> SMGKKSRVKTQKSGTGATATVSPKEILNLTSELLQKCSSPAPGPGKEWEEYVQIRTLVEKIRKKQKGLSVTFDGKREDYFPDLMKWASENGASVEGFEMVNFKEEGFGLRATRDIKAEELFLWVPRKLLMTVESAKNSVLGPLYSQDRILQAMGNIALAFHLLCERASPNSFWQPYIQTLPSEYDTPLYFEEDEVRYLQSTQAIHDVFSQYKNTARQYAYFYKVIQTHPHANKLPLKDSFTYEDYRWAVSSVMTRQNQIPTEDGSRVTLALIPLWDMCNHTNGLITTGYNLEDDRCECVALQDFRAGEQIYIFYGTRSNAE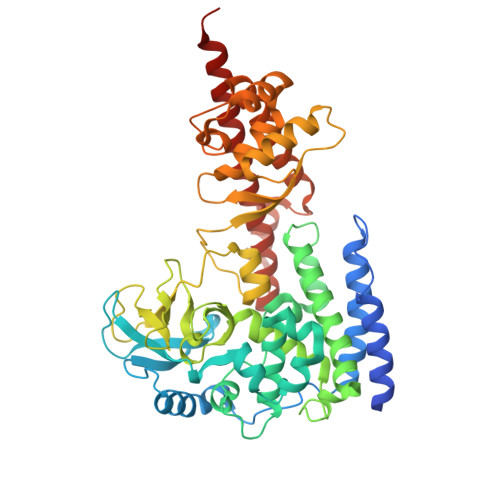FVIHSGFFFDNNSHDRVKIKLGVSKSDRLYAMKAEVLARAGIPTSSVFALHFTEPPISAQLLAFLRVFCMTEEELKEHLLGDSAIDRIFTLGNSEFPVSWDNEVKLWTFLEDRASLLLKTYKTTIEEDKSVLKNHDLSVRAKMAIKLRLGEKEILEKAVKSAAVNREYYRQQMEEKAP> MLGTGPAAATTAATTSSNVSVLQQFASGLKSRNEETRAKAAKELQHYVTMELREMSQEESTRFYDQLNHHIFELVSSSDANERKGGILAIASLIGVEGGNATRIGRFANYLRNLLPSNDPVVMEMASKAIGRLAMAGDTFTAEYVEFEVKRALEWLGADRNEGRRHAAVLVLRELAISVPTFFFQQVQPFFDNIFVAVWDPKQAIREGAVAALRACLILTTQREPKEMQKPQWYRHTFEEAEKGFDETLAKEKGMNRDDRIHGALLILNELVRISSMEGERLREEMEEITQQQLVHDKYCKDLMGFGTKPRHITPFTSFQAVQPQQSNALVGLLGYSSHQGLMGFGTSPSPAKSTLVESRCCRDLMEEKFDQVCQWVLKCRNSKNSLIQMTILNLLPRLAAFRPSAFTDTQYLQDTMNHVLSCVKKEKERTAAFQALGLLSVAVRSEFKVYLPRVLDIIRAALPPKDFAHKRQKAMQVDATVFTCISMLARAMGPGIQQDIKELLEPMLAVGLSPALTAVLYDLSRQIPQLKKDIQDGLLKMLSLVLMHKPLRHPGMPKGLAHQLASPGLTTLPEASDVGSITLALRTLGSFEFEGHSLTQFVRHCADHFLNSEHKEIRMEAARTCSRLLTPSIHLISGHAHVVSQTAVQVVADVLSKLLVVGITDPDPDIRYCVLASLDERFDAHLAQAENLQALFVALNDQVFEIRELAICTVGRLSSMNPAFVMPFLRKMLIQILTELEHSGIGRIKEQSARMLGHLVSNAPRLIRPYMEPILKALILKLKDPDPDPNPGVINNVLATIGELAQVSGLEMRKWVDELFIIIMDMLQDSSLLAKRQVALWTLGQLVASTGYVVEPYRKYPTLLEVLLNFLKTEQNQGTRREAIRVLGLLGALDPYKHKVNIGMIDQSRDASAVSLSESKSSQDSSDYSTSEMLVNMGNLPLDEFYPAVSMVALMRIFRDQSLSHHHTMVVQAITFIFKSLGLKCVQFLPQVMPTFLNVIRVCDGAIREFLFQQLGMLVSFVKSHIRPYMDEIVTLMREFWVMNTSIQSTIILLIEQIVVALGGEFKLYLPQLIPHMLRVFMHDNSPGRIVSIKLLAAIQLFGANLDDYLHLLLPPIVKLFDAPEAPLPSRKAALETVDRLTESLDFTDYASRIIHPIVRTLDQSPELRSTAMDTLSSLVFQLGKKYQIFIPMVNKVLVRHRINHQRYDVLICRIVKGYTLADEEEDPLIYQHRMLRSGQGDALASGPVETGPMKKLHVSTINLQKAWGAARRVSKDDWLEWLRRLSLELLKDSSSPSLRSCWALAQAYNPMARDLFNAAFVSCW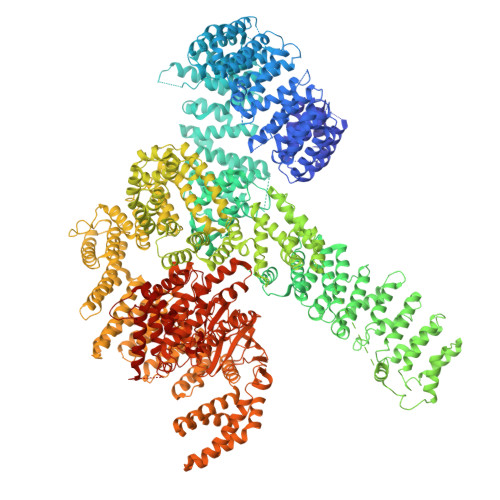SELNEDQQDELIRSIELALTSQDIAEVTQTLLNLAEFMEHSDKGPLPLRDDNGIVLLGERAAKCRAYAKALHYKELEFQKGPTPAILESLISINNKLQQPEAAAGVLEYAMKHFGELEIQATWYEKLHEWEDALVAYDKKMDTNKDDPELMLGRMRCLEALGEWGQLHQQCCEKWTLVNDETQAKMARMAAAAAWGLGQWDSMEEYTCMIPRDTHDGAFYRAVLALHQDLFSLAQQCIDKARDLLDAELTAMAGESYSRAYGAMVSCHMLSELEEVIQYKLVPERREIIRQIWWERLQGCQRIVEDWQKILMVRSLVVSPHEDMRTWLKYASLCGKSGRLALAHKTLVLLLGVDPSRQLDHPLPTVHPQVTYAYMKNMWKSARKIDAFQHMQHFVQTMQQQAQHAIATEDQQHKQELHKLMARCFLKLGEWQLNLQGINESTIPKVLQYYSAATEHDRSWYKAWHAWAVMNFEAVLHYKHQNQARDEKKKLRHASGANITNATTAATTAATATTTASTEGSNSESEAESTENSPTPSPLQKKVTEDLSKTLLMYTVPAVQGFFRSISLSRGNNLQDTLRVLTLWFDYGHWPDVNEALVEGVKAIQIDTWLQVIPQLIARIDTPRPLVGRLIHQLLTDIGRYHPQALIYPLTVASKSTTTARHNAANKILKNMCEHSNTLVQQAMMVSEELIRVAILWHEMWHEGLEEASRLYFGERNVKGMFEVLEPLHAMMERGPQTLKETSFNQAYGRDLMEAQEWCRKYMKSGNVKDLTQAWDLYYHVFRRISKQLPQLTSLELQYVSPKLLMCRDLELAVPGTYDPNQPIIRIQSIAPSLQVITSKQRPRKLTLMGSNGHEFVFLLKGHEDLRQDERVMQLFGLVNTLLANDPTSLRKNLSIQRYAVIPLSTNSGLIGWVPHCDTLHALIRDYREKKKILLNIEHRIMLRMAPDYDHLTLMQKVEVFEHAVNNTAGDDLAKLLWLKSPSSEVWFDRRTNYTRSLAVMSMVGYILGLGDRHPSNLMLDRLSGKILHIDFGDCFEVAMTREKFPEKIPFRLTRMLTNAMEVTGLDGNYRITCHTVMEVLREHKDSVMAVLEAFVYDPLLNWRLMDTNTKGNKRSRTRTDSYSAGQSVEILDGVELGEPAHKKTGTTVPESIHSFIGDGLVKPEALNKKAIQIINRVRDKLTGRDFSHDDTLDVPTQVELLIKQATSHENLCQCYIGWCPFW>[2x]MGVFTFEDEITSTVPPAKLYNAMKDADSITPKIIDDVKSVEIVEGNGGPGTIKKLTIVEDGETKFILHKVESIDEANYAYNYSVVGGVALP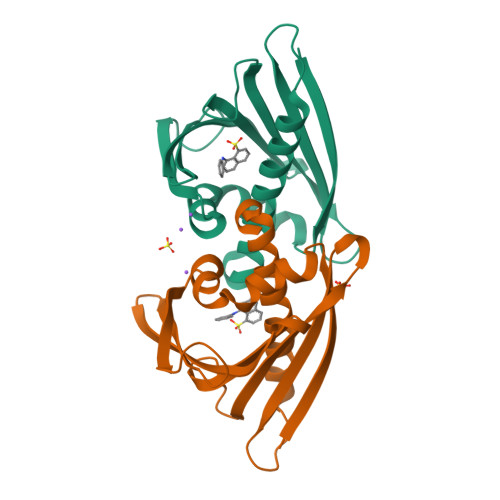PTAEKITFETKLVEGPNGGSIGKLTLKYHTKGDAKPDEEELKKGKAKGEGLFRAIEGYVLANPTQY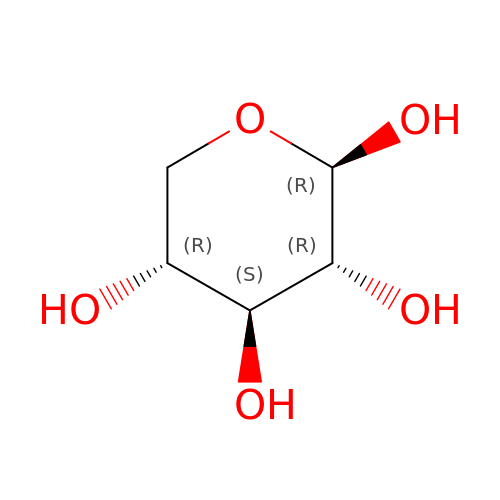beta-D-xylopyranose | C5 H10 O5 | SRBFZHDQGSBBOR-KKQCNMDGSA-N> MKIEEVR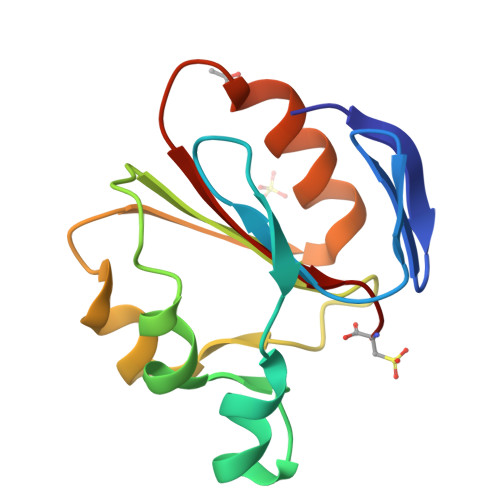FGLVKIDGKEFDHDIVIYPSGRIERRMKEISKKKHGTSHKLDPEELEKYLVEDFDVLLVGTGIYGMLSLLPESKKLVEDKEVIEKPTKEALKLLEELWGKKRILAIIHVTC> EAPRHSDWQRPTFAFEGKGAAGGHTATHHASA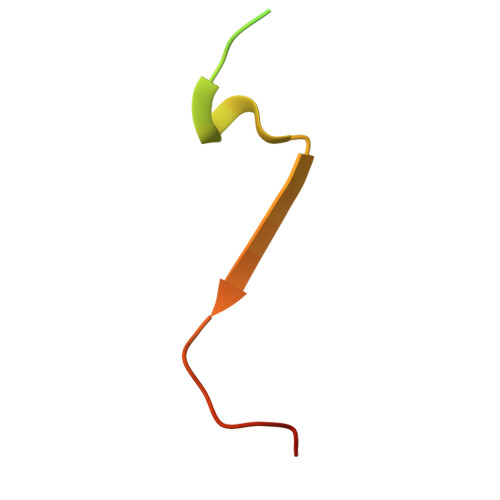APARPQPVE4-[(4R,5R)-6,7-dihydro-5H-pyrrolo[1,2-c]imidazol-5-yl]-3-fluorobenzonitrile 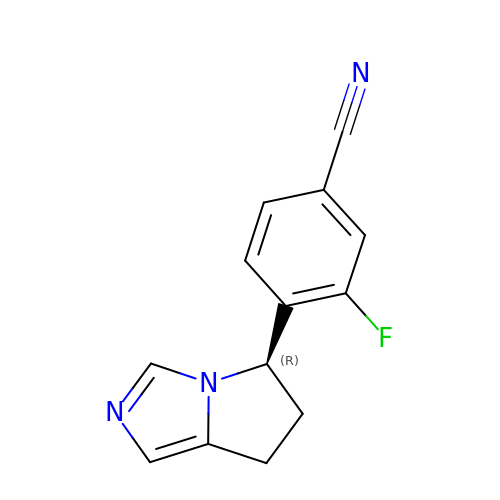| C13 H10 F N3 | USUZGMWDZDXMDG-CYBMUJFWSA-N> PFFVNRGGLPVDEATWE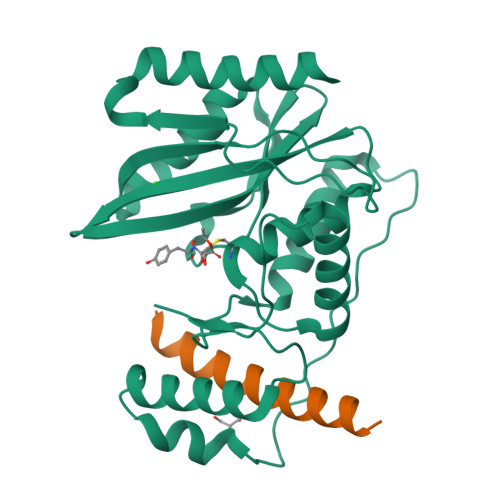RMWKHVAKIHPDGEKVAQRIRGATDLPKIPIPSVPTFQPSTPVPERLEAVQRYIRELQYNHTGTQFFEIKKSRPLTGLMDLAKEMTKEALPIKCLEAVILGIYLTNSMPTLERFPISFKTYFSGNYFRHIVLGVNFAGRYGALGMSRREDLMYKPPAFRTLSELVLDFEAAYGRCWHVLKKVKLGQSVSHDPHSVEQIEWKHSVLDVERLGRDDFRKELERHARDMRLKI;> SAQQELKQRQRAEIYALNRVMTELEQ> MHVKKYLLKGLHRLQKGPGYTYKELLVWYCDNTNTHGPKRIICEGPKKKAMWFLLTLLFAALVCWQWGIFIRTYLSWEVSVSLSVGFKTMDFPAVTICNASPFKYSKIKHLLKDLDELMEAVLERILAPELSHANATRNLNFSIWNHTPLVLIDERNPHHPMVLDLFGDNHNGLTSSSASEKICNAHGCKMAMRLCSLNRTQCT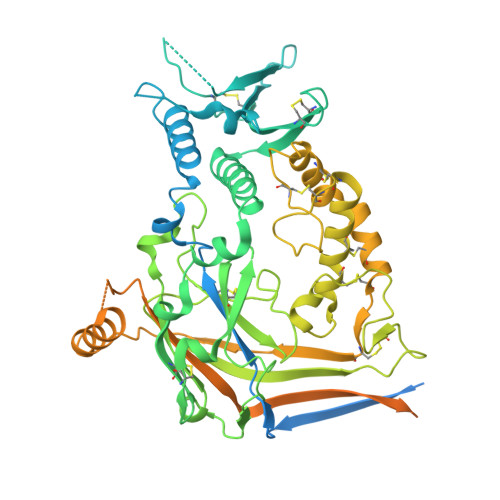FRNFTSATQALTEWYILQATNIFAQVPQQELVEMSYPGEQMILACLFGAEPCNYRNFTSIFYPHYGNCYIFNWGMTEKALPSANPGTEFGLKLILDIGQEDYVPFLASTAGVRLMLHEQRSYPFIRDEGIYAMSGTETSIGVLVDKLQRMGEPYSPCTVNGSEVPVQNFYSDYNTTYSIQACLRSCFQDHMIRNCNCGHYLYPLPRGEKYCNNRDFPDWAHCYSDLQMSVAQRETCIGMCKESCNDTQYKMTISMADWPSEASEDWIFHVLSQERDQSTNITLSRKGIVKLNIYFQEFNYRTIEESAANNIVWLLSNLGGQFGFWMGGSVLCLIEFGEIIIDFVWITIIKLVALAKSLRQRRAQASYAGPPPTVAELVEAHTNFGFQPDTAPRSPNTGPYPSEQALPIPGTPPPNYDSLRLQPLDVIESDSEGDAI9-piperazin-1-yl-4-(3,4,5-trimethoxyphenyl)-5,6-dihydro-[1]benzoxepino[5,4-c]pyridine 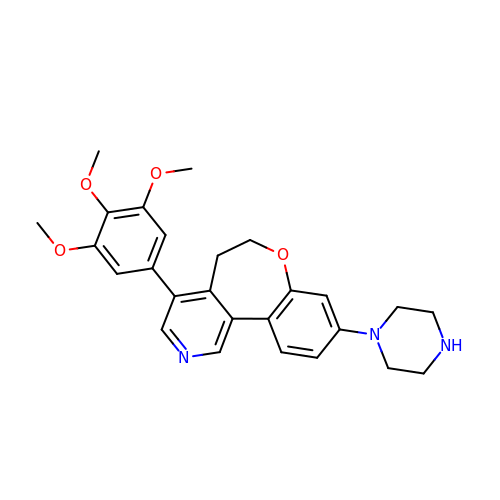| C26 H29 N3 O4 | QFFKJPJEWNRMHC-UHFFFAOYSA-N6-{[1-(anthracen-9-ylcarbonyl)piperidin-4-yl]methyl}-2-methylquinoline | C31 H28 N2 O | 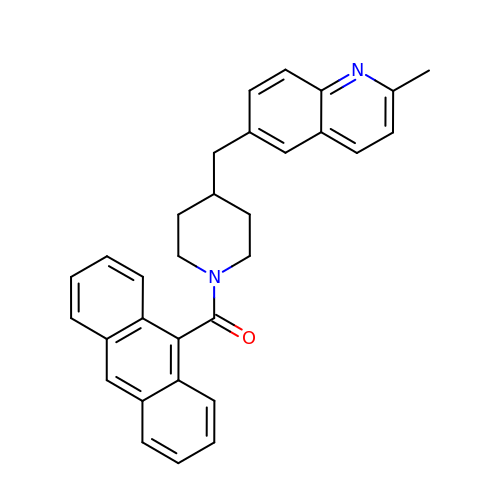FVPWEZQBGAOBRM-UHFFFAOYSA-N>[2x]MHHHHHHSTENLYFQGSSTSCNPSDMSHGYVTVKPRVRLHFVELGSGPAVCLCHGFPESWYSWRYQIPALAQAGYRVLAMDMKGYGESSAPPEIEEYCMEVLCKEMVTFLDKLGLSQAVFIGHDWGGMLVWYMALFYPERVRAVASLNTPFIPANPNMSPLESIKANPVFDYQLYFQEPGVAEAELEQNLSRTFKSLFRASDESVLSMHKVCEAGGLFVNS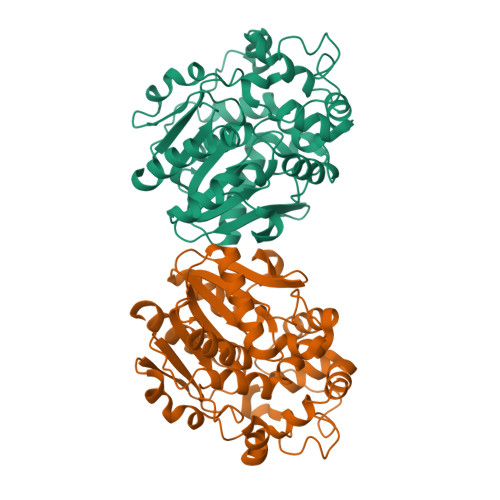PEEPSLSRMVTEEEIQFYVQQFKKSGFRGPLNWYRNMERNWKWACKSLGRKILIPALMVTAEKDFVLVPQMSQHMEDWIPHLKRGHIEDCGHWTQMDKPTEVNQILIKWLDSDARNPPVVSKM Transportin 3 (TNPO3) is a nuclear import receptor known for its broad substrate specificity, often recognizing arginine-serine (SR/RS) repeat-rich nuclear localization signals (NLS) in SRSF proteins. TNPO3 consists of 20 pairs of tandemly repeated alpha helices known as HEAT repeats, named after the proteins in which they were initially discovered. It adopts a C-shaped structure enabling it to interact with the nuclear pore complex (NPC) on its outer surface and with cargos as well as RanGTP on its inner surface. One such example is the cold-inducible RNA-binding protein (CIRBP), which contains a non-classical RSY-NLS.

We next aimed to gain insight into the structural basis for TNPO3 recognition of RSY-NLS and obtained crystals of TNPO3 C511A bound to CIRBPRSY that diffracted X-rays to 2.94 Å resolution. TNPO3 forms a dimer in the asymmetric unit of the crystal structure, as previously observed, and CIRBPRSY was bound to each monomer. For the CIRBPRSY peptide, only 14 residues (amino acids 158–171) from the full CIRBP fragment (amino acids 138–172) could be modeled unambiguously. These residues form two short helices, each containing a single turn (residues 159–163 and 166–170). Inspection of the TNPO3-CIRBPRSY crystal structure revealed that the binding site of CIRBPRSY on TNPO3 is located between HEAT repeats 14 and 17 and involves more than 15 amino-acids. TNPO3-CIRBP complex formation is driven by several electrostatic interactions via the charged side chains of CIRBP R161 and TNPO3 D747/D751 as well as CIRBP D165 and TNPO3 R667/R671. Importantly, three CIRBP tyrosines (Y167, Y160, and Y164) are engaged in a network of interactions including hydrogen bonds (with TNPO3 S705, D751 and E660), π stacking of CIRBP Y164 with TNPO3 Y702 and cation-π interactions of CIRBP Y167 and TNPO3 R758. Unlike the canonical ligands pSRSF1 and pCPSF6, which lacks a helix at the binding site, CIRBPRSY forms two short helices between S159-S163 and S166-H170, respectively. To accommodate the loop connecting these helices, the TNPO3 ligand-binding cavity opened up which is visible by a movement of TNPO3 helices 14 and 15. Recognition of the CIRBP tyrosines compensates the lack of phosphorylation via structural arrangements of the TNPO3 binding surface and generation of binding pockets accommodating tyrosine residues.

>MEGAKPTLQLVYQAVQALYHDPDPSGKERASFWLGELQRSVHAWEISDQLLQIRQDVESCYFAAQTMKMKIQTSFYELPTDSHASLRDSLLTHIQNLKDLSPVIVTQLALAIADLALQMPSWKGCVQTLVEKYSNDVTSLPFLLEILTVLPEEVHSRSLRIGANRRTEIIEDLAFYSSTVVSLLMTCVEKAGTDEKMLMKVFRCLGSWFNLGVLDSNFMANNKLLALLFEVLQQDKTSSNLHEAASDCVCSALYAIENVETNLPLAMQLFQGVLTLETAYHMAVAREDLDKVLNYCRIFTELCETFLEKIVCTPGQGLGDLRTLELLLICAGHPQYEVVEISFNFWYRLGEHLYKTNDEVIHGIFKAYIQRLLHALARHCQLEPDHEGVPEETDDFGEFRMRVSDLVKDLIFLIGSMECFAQLYSTLKEGNPPWEVTEAVLFIMAAIAKSVDPENNPTLVEVLEGVVRLPETVHTAVRYTSIELVGEMSEVVDRNPQFLDPVLGYLMKGLAEKPLASAAAKAIHNICSVCRDHMAQHFNGLLEIARSLDSFLLSPEAAVGLLKGTALVLARLPLDKITECLSELCSVQVMALKKLLSQEPSNGISSDPTVFLDRLAVIFRHTNPIVENGQTHPCQKVIQEIWPVLSETLNKHRADNRIVERCCRCLRFAVRCVGKGSAALLQPLVTQMVNVYHVHQHSCFLYLGSILVDEYGMEEGCRQGLLDMLQALCIPTFQLLEQQNGLQNHPDTVDDLFRLATRFIQRSPVTLLRSQVVIPILQWAIASTTLDHRDANCSVMRFLRDLIHTGVANDHEEDFELRKELIGQVMNQLGQQLVSQLLHTCCFCLPPYTLPDVAEVLWEIMQVDRPTFCRWLENSLKGLPKETTVGAVTVTHKQLTDFHKQVTSAEECKQVCWALRDFTRLFR[2x];>[3x]SRDYYSSRSQSGGYSDRSSGGSYRDSYDSYATHNE>[8x]GSHMVIRATTWKDLDLPRLQHLIQSSFRRTLIPHYFETTPLLRAY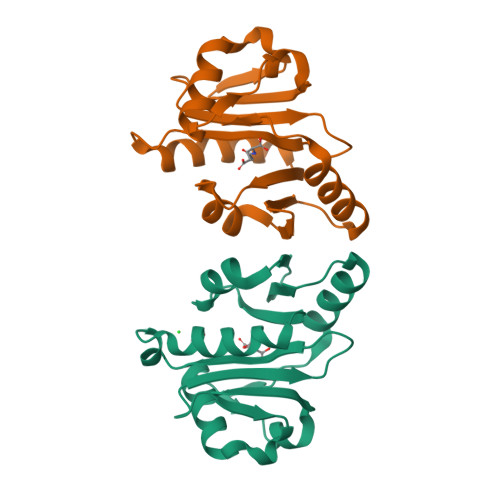VSENYRAAVILTKLGNVPYLDKFAVLDDAQGEGLGRAVWSIMREETPQLFWRSRHNNQANAFYYAESDGYYKQDHWKIFWNGLHHFQQIQQCVAHCTQHPPTLID> MSYPLSKFH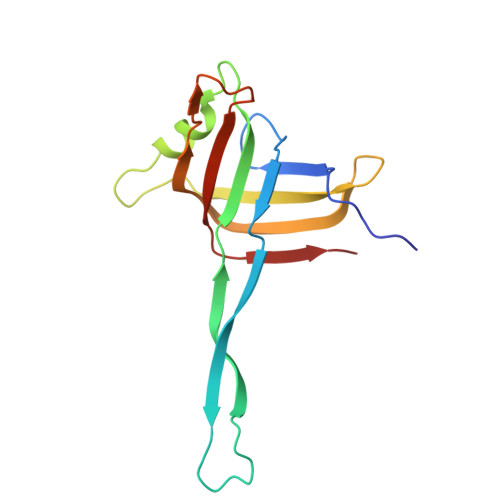FSVEWGGTKIGFTEVSGLDLETEIIEYRHGASPEYSKIKMPGMQKFSNITLKRGTFKSDNEYFQWYNTINLNKVERRDLTISLLNEEHEPVVTWKVKNAWPLKVQSTDLKGDGNEVAIESMELAHEGLVIQNE> MQFFKTLAALVSCISFVLAYVAQDVHVSFPSTAGKSRVMIGKVEPRIGIDETVPTTITVEDPNEVIQVNFAIESTNKPFQNTLLIGLPNKNLEMAFEPEIKDNGKLSMYKYRIDLAKLDAALLQEASRSPEPIKATLILASSTAKPKENLFREILQLNLNFDVDHSDSSLVDKFGIKPEIHHIFHAEPKRVAKPIAVIFVLIIFITILSLIVTWLNSCAAAFNNIPTGVTAVYFLGFIATIVGFEVIFARY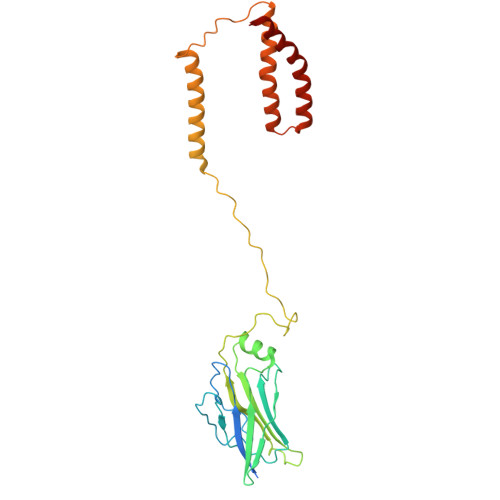YLGTSIFETLFSSLYLGAPGLLTSTKFLRSFG>AGHML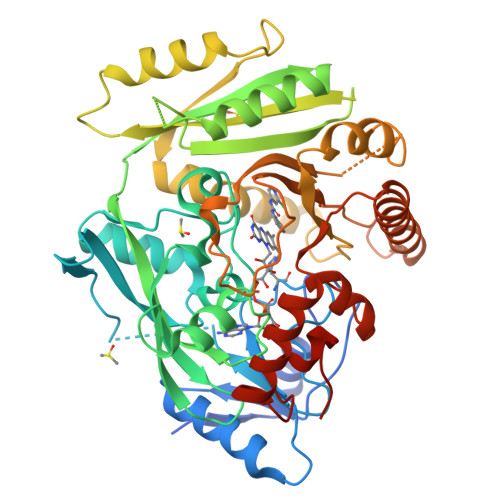PVEPPAELLQLGGGDVGGGRLSVDASDIAEASRDFGGVARAEPMAVFHPRAAGDVAGLVGAAFRSARGFRVSARGHGHSISGQAQAAGGVVVDMSRGRGPGAAVARALPVHSAALGGHYVDVWGGELWVDVLNWTLSHGGLAPRSWTDYLYLSVGGTLSNAGISGQAFHHGPQISNVYELDVVTGKGEVVTCSETENPDLFFGVLGGLGQFGIITRARIALERAPKRVRWIRALYSNFSEFTADQERLISLGSGGGRRFDYVEGFVVAAEGLINNWRSSFFSPQNPVKLTSLKHHSSVLYCLEVTKNYDDETAGSVDQDVDTLLGELNFLPGTVFTTDLPYVDFLDRVHKAELKLRAKGMWEVPHPWLNLFVPASRIADFDRGVFRGVLGGRTAGAGGPVLIYPMNKHKWDPRSSAVTPDEEVFYLVAFLRSALPGAPESLEALARQNQRILDFCAGTGIGAKQYLPGHKARHEWAEHFGAARWDRFARLKAEFDPRAILAAGQGIFRPPGSPALAADS[2x]> GMTQRSLADIQFQTTLEGVTPAQLGGFFEGWPNPPTPETLWRILDRAAVFVLARTPDGQVIGFVNALSDGILAASIPLLEVQAGW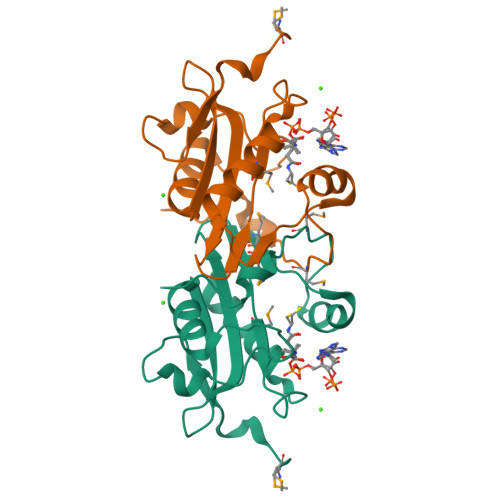RSLGLGSELMRRVLTELGDLYMVDLSCDDDVVPFYERLGLKRANAMFLRRYDNQAGIPAE> GGLTQRVADGTVSATKSLFYRQIKTLHLDIRAREAINTSAAGIPLSVVVRIYQLKDNRSFDSADYQALFTGDNEILAGDIIAQK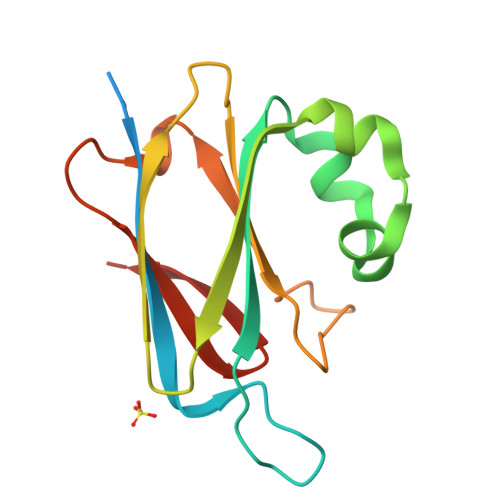DVWLQPGGSVAVDMPLDDAAKFTGVAAMFLEPDQKKNTWRVVLGRDELEPDTPRLIEVSGNTLTLLPVKDK(1S,2S,3R,4S,6R)-4,6-diamino-3-{[(2S,3R)-3-amino-6-(aminomethyl)-3,4-dihydro-2H-pyran-2-yl]oxy}-2-hydroxycyclohexyl 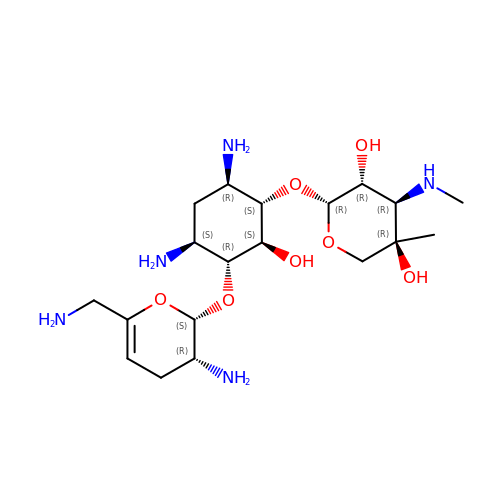3-deoxy-4-C-methyl-3-(methylamino)-beta-L-arabinopyranoside | C19 H37 N5 O7 | URWAJWIAIPFPJE-YFMIWBNJSA-N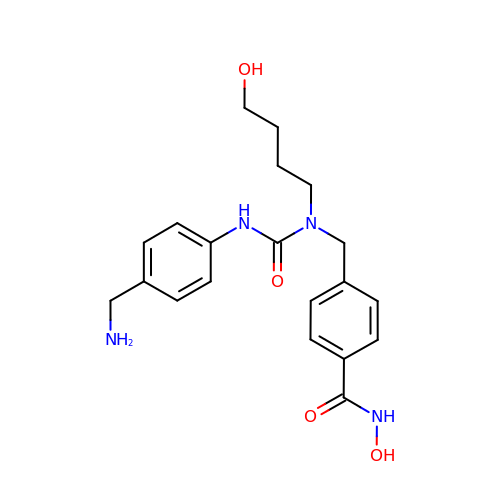4-[[[4-(aminomethyl)phenyl]carbamoyl-(4-oxidanylbutyl)amino]methyl]-~{N}-oxidanyl-benzamide | C20 H26 N4 O4 | VTRGFHYHEAEHGS-UHFFFAOYSA-N> MRVNNCLTPEELEAYGISDVHDIVYNPSYDLLYQEELDPSLTGYERGVLTNLGAVAVDTGIFTGRSPKDKYIVRDDTTRDTFWWADKGKGKNDNKPLSPETWQHLKGLVTRQLSGKRLFVVDAFCGANPDTRLSVRFITEVAWQAHFVKNMFIRPSDEELAGFKPDFIVMNGAKCTNPQWKEQGLNSENFVAFNLTERMQLIGGTWYGGEMKKGMFSMMNYLLPLKGIASMHCSANVGEKGDVAVFFGLSGTGKTTLSTDPKRRLIGDNEHGWDDDGVFNFEGGCYAKTIKLSKEAEPEIYNAIRRDALLENVTKREDGTIDFDDGSKTENTRVSYPIYHIDNIVKPVSKAGHATKVIFLTADAFGVLPPVSRLTADQTQYHFLSGFTAKLAG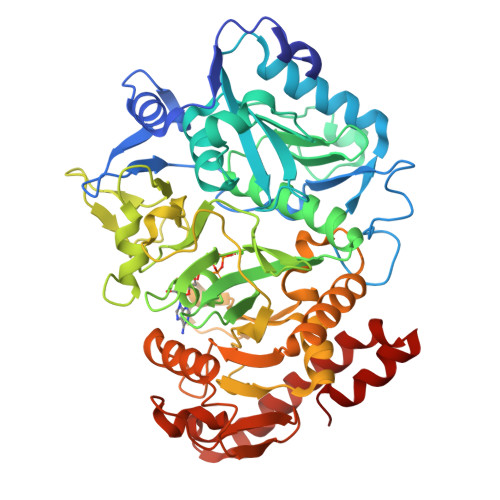TERGITEPTPTFSACFGAAFLSLHPTQYAEVLVKRMQAAGAQAYLVNTGWNGTGKRISIKDTRAIIDAILNGSLDNAETFTLPMFNLAIPTELPGVDTKILDPRNTYASPEQWQEKAETLAKLFIDNFDKYTDTPAGAALVAAGPKL> MISDEQLNSLAITFGIVMMTLIVIYHAV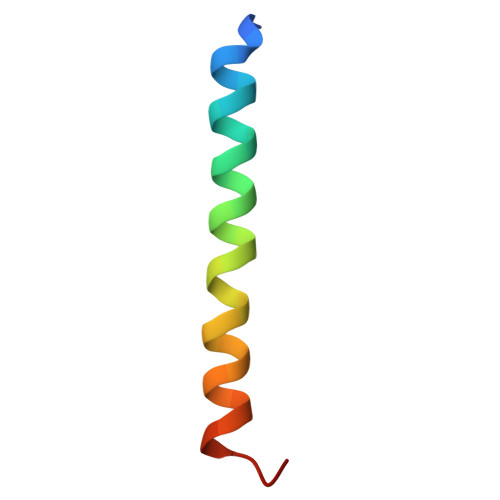DSTMSPKN>[2x]SNASQGRACLSKAELTADLI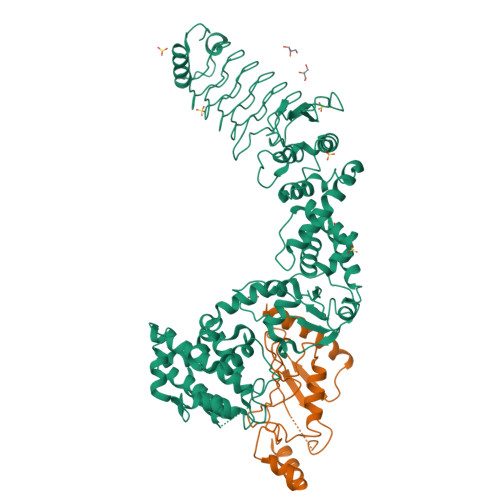WLSANRTGEESAEELNYSGCDLSGLSLVGLNLSSVNFSGAVLDDTDLRMSDLSQAVLENCSFKNSILNECNFCYANLSNCIIRALFENSNFSNSNLKNASFKGSSYIQYPPILNEADLTGAIIIPGMVLSGAILGDVKELFSEKSNTINLGGCYIDLSDIQENILSVLDNYTKSNKSILLTMNTSDDKYNHDKVRAAEELIKKISLDELAAFRPYVKMSLADSFSIHPYLNNANIQQWLEPICDDFFDTIMSWFNNSIMMYMENGSLLQAGMYFERHPGAMVSYNSSFIQIVMNGSRRDGMQERFRELYEVYLKNEKVYPVTQQSDFGLCDGSGKPDWDDDSDLAYNWVLLSSQDDGMAMMCSLSHMVDMLSPNTSTNWMSFFLYKDGEVQNTFGYSLSNLFSESFPIFSIPYHKAFSQNFVSGILDILISDNELKERFIEALNSNKSDYKMIADDQQRKLACVWNPFLDGWELNAQHVDMIMGSHVLKDMPLRKQAEILFCLGGVFCKYSSSDMFGTEYDSPEILRRYANGLIEQAYKTDPQVFGSVYYYNDILDRLQGRNNVFTCTAVLTDMLTEHAKESFPEIFSLYYPVAWR;>[2x]GSMAASRRLMKELEEIRKCGMKNFRNIQVDEANLLTWQGLIVPDNPPYDKGAFRIEINFPAEYPFKPPKITFKTKIYHPNIDEKGQVCLPVISAENWKPATKTDQVIQSLIALVNDPQPEHPLRADLAEEYSKDRKKFCKNAEEFTKKYGEKRPVD> HMIHEDFCSVCRKSGQLLMCDTCSRVYHLDCLDPPLKTI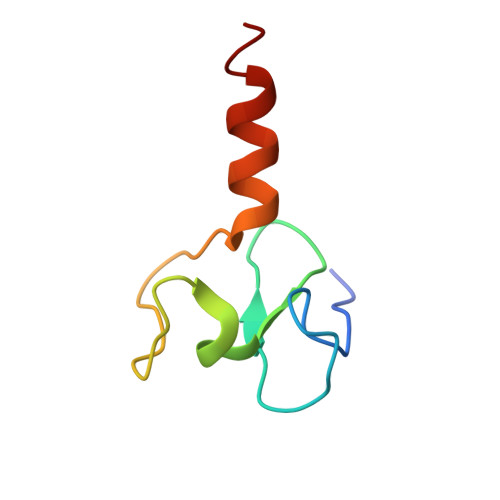PKGMWICPRCQDQMLKKEEAI>[2x]MSSGKKPVKVKTPAGKE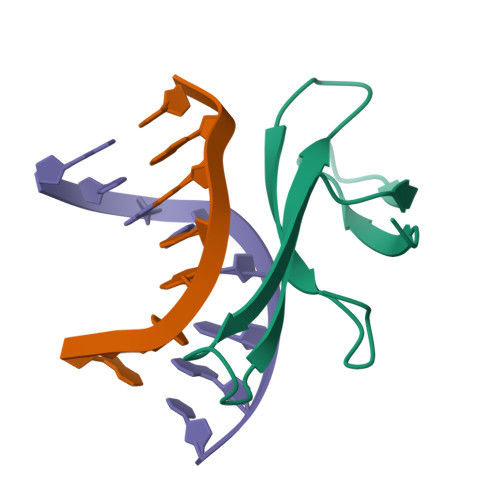AELVPEKVWAMAPKGRKGVKIGLFKDPETGKYFRHKLPDDYPI>[2x]DYKDEMYSFEQAITQLFQQLSLSIPDTIEPVIGVKVGEFACHITEH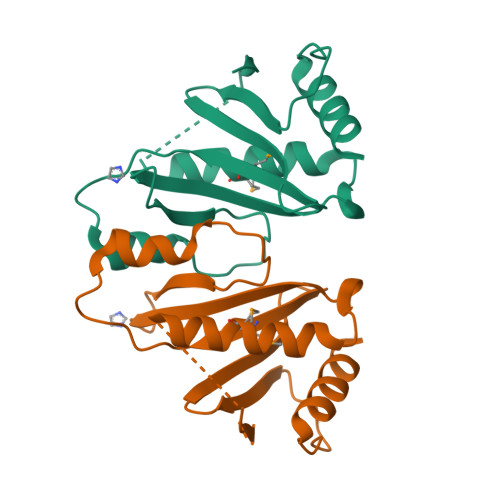PVGQILMFTLPSLDNNDEKETLLSHNIFSQDILKPILSWDEVGGHPVLWNRQPLNSLDNNSLYTQLEMLVQGAERLQTSSLISPPRSFSHHHHHH>[2x]MERKISRIHLVSEPSITHFLQVSWEKTLESGFVITLTDGHSAWTGTVSESEISQEADDMAMEKGKYVGELRKALLSGAGP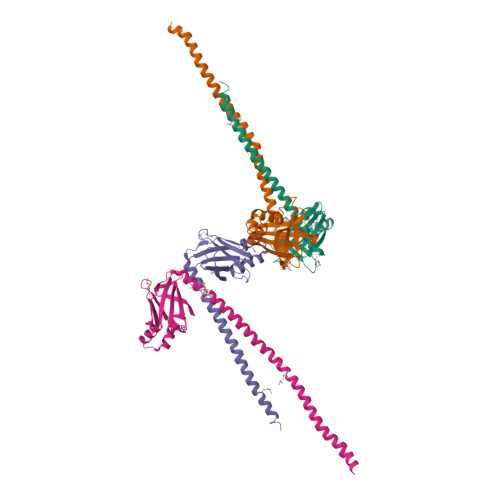ADVYTFNFSKESCYFFFEKNLKDVSFRLGSFNLEKVENPAEVIRELICYCLDTTAENQAKNEHLQKENERLLRDWNDVQGRFEKCVSAKEALETDLYKRFILVLNEKKTKIRSLHNKLLNAAQ> GSHMVLKFPKQQLPPKKKRRVGTTVHCDYLNRPHKSIHRRRTDPMVTLSSILESIINDMRDLPNTYPFHTPVNAKV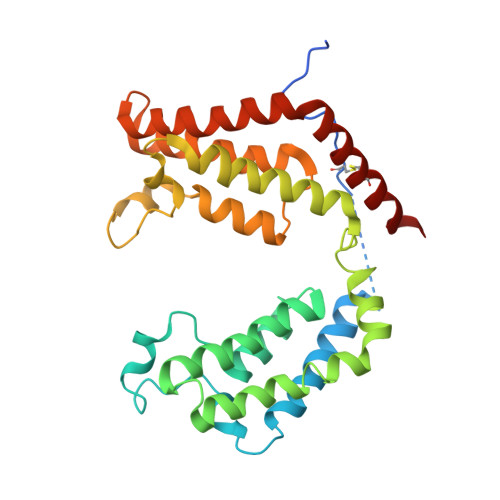VKDYYKIITRPMDLQTLRENVRKRLYPSREEFREHLELIVKNSATYNGPKHSLTQISQSMLDLCDEKLKEKEDKLARLEKAINPLLDDDDQVAFSFILDNIVTQKMMAVPDSWPFHHPVNKKFVPDYYKVIVNPMDLETIRKNISKHKYQSRESFLDDVNLILANSVKYNGPESQYTKTAQEIVNVCYQTLTEYDEHLTQLEKDICTAKEAALEEA>[2x]MASTDYHVDLTNCDREPIHIPGYIQPHGCLIACDNAMRMVLRHSENCGELLGLEGDLNGRTAEDVLGKRLVHDLRNALTVTGKTTRPAMLPAMETSDGRSFDISLHRYKSTTIIEFEPSDSDTQPLGTARKMVDRIREADSVESLISRTTRLVKATLGYDRVLIYRFEEDGAGKVVSEAKQPELESFLGQYFPASDIPQQARALYLKNTLRIISDASGTPIPVLPAVDVSGEPLDLSYAHLRNFSPIHCEYLRNMGVAASMSISVIVDDALWGLIVCHHCSPRVLSMPVRIAAAMFGEFF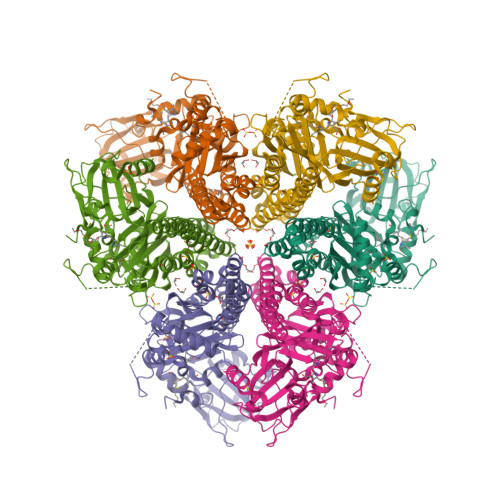SMFLQVLKQKRRLDTINHAHAALDRFLRLAAHRANLEELLVDSFQDFARLIPCDGVGLWVGNNWHGHGATPPHDAIPRLARFVASVSEGRVWATHALSQAIPEAEIYADTAAGMLAIPISQVKSDYLLFFRKEIVQNLNWAGNPEKSYETGPMGDRLTPRKSFAIWKESVRLQAQPWSEADREIAETARIALVGVAFHHSELMAGLEYK> DMPRPTGLAADIRWTAYGVPHIRAKDERGLGYGIGYAYARDNACLLAEEIVTARGERARYFGSEGKSSAELDNLPSDIFYAWLNQPEALQAFWQAQTPAVRQLLEGYAAGFNRFLREADGKTTSCLGQPWLRAIATDDLLRLTRRLLVEGGVGQFA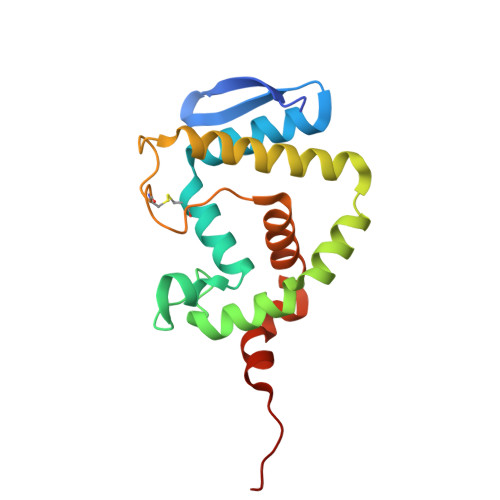DALVAAAPPGAEKV> GLPTMNTPGSTQFLTSDDFQSPCALPQFDVTPSMNIPGEVKNLMEIAEVDSVVPVNNVQDTTDQMEMFRIPVTINAPLQQQVFGLRLQPGLDSVFKHTLLGEILNYYAHWSGSMKLTFVFCGSAMATGKFLIAYSPPGANPPKTRKDAML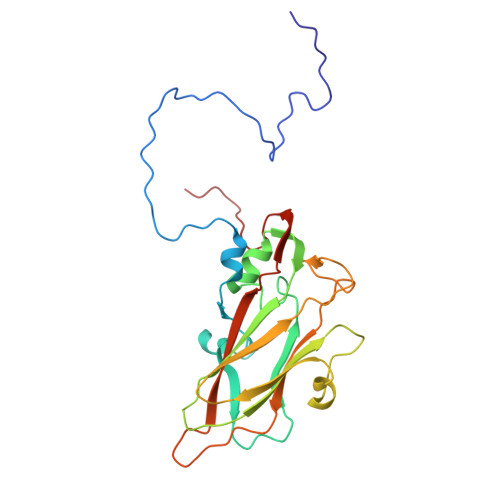GTHIIWDIGLQSSCVLCVPWISQTHYRLVQQDEYTSAGYVTCWYQTGMIVPPGTPNSSSIMCFASACNDFSVRMLRDTPFISQDNKLQ>[3x]DLVNLLRCQEGPRNCRELLSQGATLSGWYHLCLPEG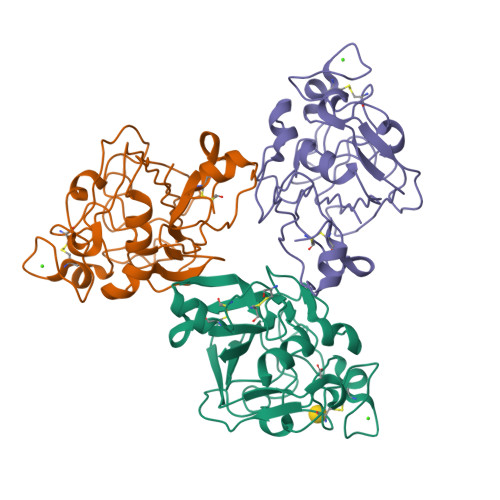RALPVFCDMDTEGGGWLVFQRRQDGSVDFFRSWSSYRAGFGNQESEFWLGNENLHQLTLQGNWELRVELEDFNGNRTFAHYATFRLLGEVDHYQLALGKFSEGTAGDSLSLHSGRPFTTYDADHDSSNSNCAVIVHGAWWYASCYRSNLNGRYAVSEAAAHKYGIDWASGRGVGHPYRRVRMMLR> AAPNLAGAVEFSDVKTLLKEWITTISDPMEEDILQVVRYCTDLIEEKDLEKLDLVIKYMKRLMQQSVESVWNMAFDFILDNVQVVLQQTYGSTLKVT;> SFFDKKRSER;> MTTLTRQDLNFGQVVADVLSEFLEVAVHLILYVREVYPVGIFQKRKKYNVPVQMSCHPELNQYIQDTLHCVKPLLEKNDVEKVVVVILDKEHRPVEKFVFEITQPPLLSINSDSL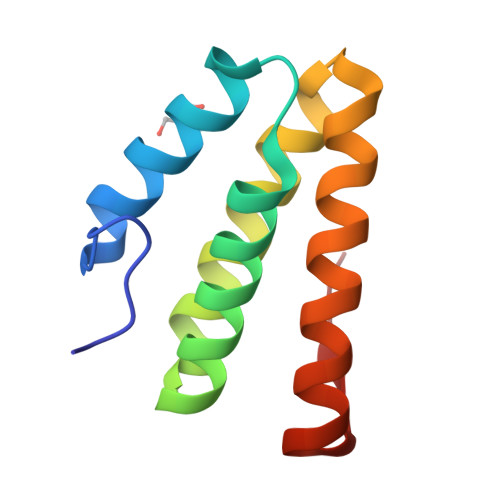LSHVEQLLAAFILKISVCDAVLDHNPPGCTFTVLVHTREAATRNMEKIQVIKDFPWILADEQDVHMHDPRLIPLKTMTSDILKMQLYVEERAHKN;> GSFTPRTAHILKPLMSPPSREEIVATLLDH>GSHMSKAFDLVVIGAGSGGLEAGWNAATLYGKRVAVVDVQTSHGPPFYAALGGTCVNVGCVPKKLMVTGAQYMDHLRESAGFGWEFDGSSVKANWKKLIAAKNEAVLDINKSYEGMFNDTEGLDFFLGWGSLESKNVVVVRETADPKSAVKERLQADHILLATGSWPQMPAIPGIEHCISSNEAFYLPEPPRRVLTVGGGFISVEFAGIFNAYKPPGGKVTLCYRNNLILRGFDETIREEVTKQLTANGIEIMTNENPAKVSLNTDGSKHVTFESGKTLDVDVVMMAIGRIPRTNDLQLGNVGVKLTPKGGVQVDEFSRTNVPNIYAIGDITD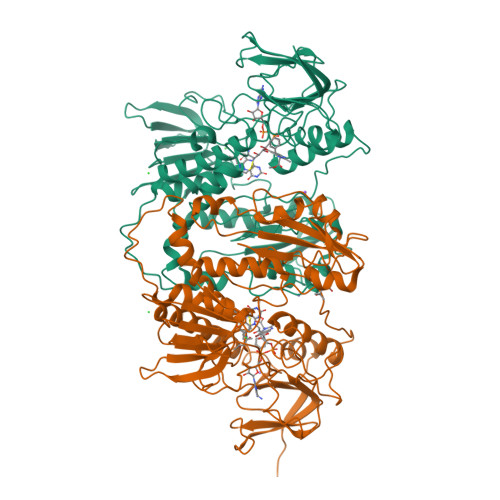RLMLTPVAINEGAALVDTVFGNKPRKTDHTRVASAVFSIPPIGTCGLIEEVAAKEFEKVAVYMSSFTPLMHNISGSKYKKFVAKIVTNHSDGTVLGVHLLGDGAPEIIQAVGVCLRLNAKISDFYNTIGVHPTSAEELCSMRTPSYYYVKGEKMEKLPDSNL[4x]> MEYEDLELITIWPSPTKNKLCQFIKQNLSKEHVVTQLFFIDATSSFPLSQFQKLVPPTLPENVRIYENIRINTCLDLEELSAITVKLLQILSMNKINAQRGTEDAVTEPLKI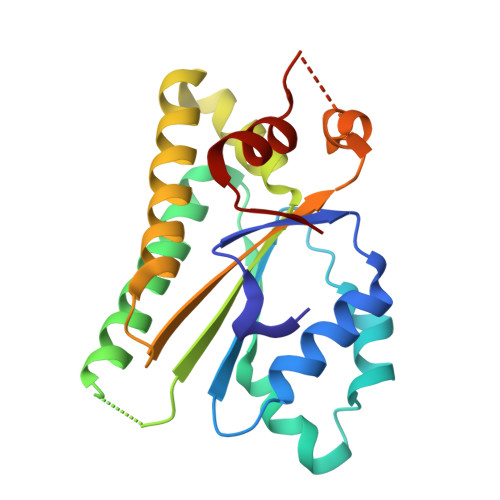ILYINGLEVMFRNSQFKSSPQRSHELLRDTLLKLRVMGNDENENASIRTLLEFPKEQLLDYYLKKNNNTRTSSVRSKRRRIKNGDSLAEYIWKYYADSLFE>[8x]GMMSNLYHDNTITVA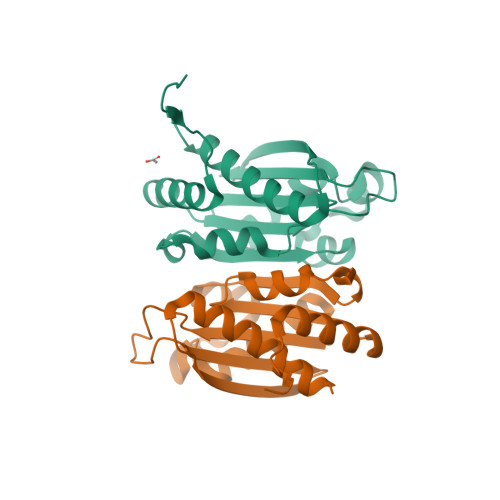ELTKKLASRLIDAGLRLTTAESCTGGKLSVALCAEENTADFYDVGLVVFSDSAKERILGVSPETLARFTAVSEQTVTEMAASIRDIAQADVSIAISGYAGPEGGEDGTAAGTVCFAWNIGGKTETSRVLFSGDCQDVVEKAVHYSLAELVTKLSG>MKLFTGLVFCSLVLGVSSEWYSFLGEAAQGAWDMWRAYSDMREANYIGADKYFHARGNYDAAQRGPGGAWAAKVISDARENSQRVTDFFRHGNSGHGAEDSKADQEANEWGRSGKDPNHYRPEGLPDKY[10x]

Specifically, AA amyloidosis represents a systemic disease characterized by the deposition of misfolded serum amyloid A protein (SAA) in multiple organs. This 12–14 kDa remarkably conserved apo-lipoprotein acts as molecular mop to remove membrane debris and lipid degradation products from inflammatory injury sites. As part of the host innate response to inflammation, acute-phase SAA is secreted by the liver to increase serum levels up to 1000-fold. Chronic inflammation leads to sustained increased SAA concentrations, to an extent that macrophages reportedly fail to prevent proteolysis-resistant oligomers during lysosomal degradation.

Herein, we present the cryo-EM structure of fibrils extracted post-mortem from the diseased kidney of a DSH cat with systemic AA amyloidosis, deceased in a shelter with extreme disease prevalence. About 65k from initially 380k segments were refined with C2 symmetry, a left-handed twist angle of 1.3° and a helical rise of 4.9 Å to yield a final map with a nominal resolution of 3.3 Å, as estimated from half-map Fourier shell correlation curves (FSC). The fibril structure is composed of two identical proto-filaments, and exhibits the cross-β architecture characteristic of amyloid. The polypeptide of each proto-filament comprises 11 β-strands between residue positions 19 and 94 and adopts an extended hairpin structure. A central β-arch between residues Asp-50 and Arg-64 links two ~25 residue long meandering tails that stick together via side chain contacts. A noteworthy feature following the β-arch is an unusual backbone bulge adopted by the P66GGAW70 segment comprising Pro-66 modeled as cis-isomer, in contrast to the trans-Proline residues in mouse and human AA amyloid. In the assembled fibril, the N-terminal tails are surface-exposed at the edges, while the C-terminal tails are buried facing each other. At the intra-protomer interface, the edge-tail of rung layer (i) contacts the face-tails (i-1) to (i + 2), creating four hydrophobic clusters, four ionic locks and additional H-bond interactions. On the other side, at the inter-protomer interface, the face-tail (i) contacts four rung layers of the adjacent proto-filament, creating two hydrophobic clusters, four ionic locks and two additional H-bond interactions. The higher dissociation cost is mainly caused by the eight-residue insert that increases fibril core mass and enlarges the buried surface area by ~2000 Å2.> PISPIETVPVKLKPGMDGPKVKQWPLTEEKIKALVEICTEMEKEGKISKIGPENPYNTPVFAIKKKDSTKWRKLVDFRELNKRTQDFWEVQLGIPHPAGLKKKKSVTVLDVGDAYFSVPLDEDFRKYTAFTIPSINNETPGIRYQYNVLPQGWKGSPAIFQSSMTKILEPF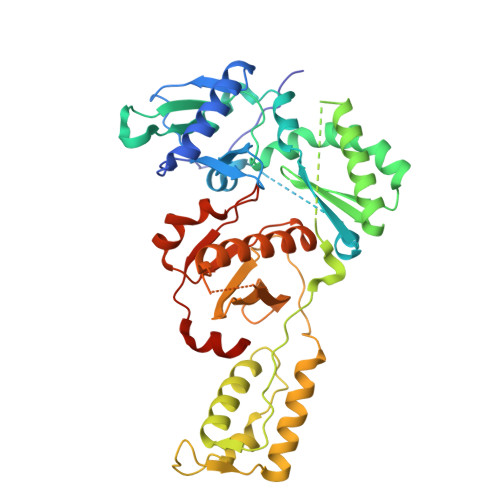RKQNPDIVIYQYVDDLYVGSDLEIGQHRTKIEELRQHLLRWGLTTPDKKHQKEPPFLWMGYELHPDKWTVQPIVLPEKDSWTVNDIQKLVGKLNWASQIYPGIKVRQLSKLLRGTKALTEVIPLTEEAELELAENREILKEPVHGVYYDPSKDLIAEIQKQGQGQWTYQIYQEPFKNLKTGKYARMRGAHTNDVKQLTEAVQKITTESIVIWGKTPKFKLPIQKETWETWWTEYWQATWIPEWEFVNTPPLVKLWYQLEKEPIVGAETF>[2x]MGSSHHHHHHSSGLVPRGSHMTGRQKARGAATRARQKQRASLETMDKAVQRFRLQNPDLDSEALLTLPLLQLVQKLQSGELSPEAVFF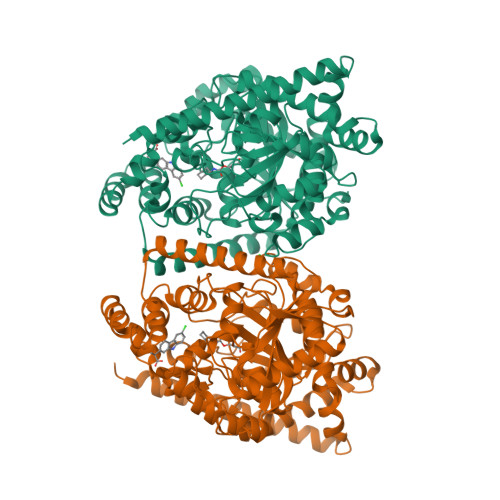TYLGKAWEVNKGTNCVTSYLTDCETQLSQAPRQGLLYGVPVSLKECFSYKGHDSTLGLSLNEGMPSESDCVVVQVLKLQGAVPFVHTNVPQSMLSFDCSNPLFGQTMNPWKSSKSPGGSSGGEGALIGSGGSPLGLGTDIGGSIRFPSAFCGICGLKPTGNRLSKSGLKGCVYGQTAVQLSLGPMARDVESLALCLKALLCEHLFTLDPTVPPLPFREEVYRSSRPLRVGYYETDNYTMPSPAMRRALIETKQRLEAAGHTLIPFLPNNIPYALEVLSAGGLFSDGGRSFLQNFKGDFVDPCLGDLILILRLPSWFKRLLSLLLKPLFPRLAAFLNSMRPRSAEKLWKLQHEIEMYRQSVIAQWKAMNLDVLLTPMLGPALDLNTPGRATGAISYTVLYNCLDFPAGVVPVTTVTAEDDAQMELYKGYFGDIWDIILKKAMKNSVGLPVAVQCVALPWQEELCLRFMREVEQLMTPQHHHHHH> MGVTSNVVLVSGEGERFTVDKKI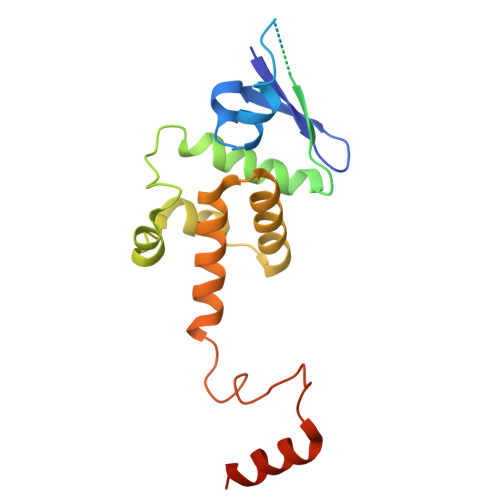AERSLLLKNYLNDMHDSNLQNNSDSESDSDSETNHKSKDNNNGDDDDEDDDEIVMPVPNVRSSVLQKVIEWAEHHRDSNFPDEDDDDSRKSAPVDSWDREFLKVDQEMLYEIILAANYLNIKPLLDAGCKVVAEMIRGRSPEEIRRTFNIVNDFTPEEEAAIRRENEWAEDRGS> MGSSHHHHHHSSGLVPRGSHMARMAPQEQAVSQVMEKQSNNNNSDVIFRSKLPDIYIPNHLSLHDYIFQNISEFATKPCLINGPTGHVYTYSDVHVISRQIAANFHKLGVNQNDVVMLLLPNCPEFVLSFLAASFRGATATAANPFFTPAEIAKQAKASNTKLIITEARYVDKIKPLQNDDGVVIVCIDDNESVPIPEGCLRFTELTQSTTEASEVIDSVEISPDDVVALPYSSGTTGLPKGVMLTHKGLVTSVAQQVDGENPNLYFHSDDVILCVLPMFHIYALNSIMLCGLRVGAAILIMPKFEINLLLELIQRCKVTVAPMVPPIVLAIAKSSETEKYDLSSIRVVKSGAAPLGKELEDAVNAKFPNAKLGQGYGMTEAGPVLAMSLGFAKEPFPVKSGACGTVVRNAEMKIVDPDTGDSLSRNQPGEICIRGHQIMKGYLNNPAATAETIDKDGWLHTGDIGLIDDDDELFIVDRLKELIKYKGFQVAPAELEALLIGHPDITDVAVVAMKEEAAGEVPVAFVVKSKDSELSEDDVKQFVSKQVVFYKRINKVFFTESIPKAPSGKILRKDLRAKLANGLGSGMASVEEFRNAQRAKGPATILAIGTATPDHCVYQSDYADYYFK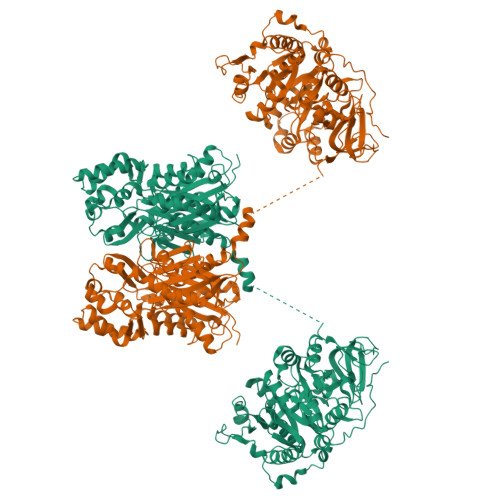VTKSEHMTALKKKFNRICDKSMIKKRYIHLTEEMLEEHPNIGAYMAPSLNIRQEIITAEVPKLGKEAALKALKEWGQPKSKITHLVFCTTSGVEMPGADYKLANLLGLEPSVRRVMLYHQGCYAGGTVLRTAKDLAENNAGARVLVVCSEITVVTFRGPSEDALDSLVGQALFGDGSAAVIVGSDPDISIERPLFQLVSAAQTFIPNSAGAIAGNLREVGLTFHLWPNVPTLISENVEKCLTQAFDPLGISDWNSLFWIAHPGGPAILDAVEAKLNLDKKKLEATRHVLSEYGNMSSACVLFILDEMRKKSLKGERATTGEGLDWGVLFGFGPGLTIETVVLHSIPMVTN> MKKHHHHHHGPEPTVEDVISQVARAHREIFTYAHDKLGSSPGNFNANHASGSPYPHGRSGRTVQEIWEDFSMSFTPAVREVVEFAKHIPGFRDLSQH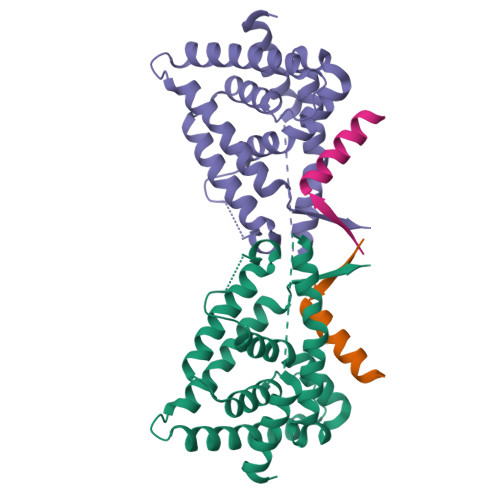DQVTLLKAGTFEVLMVRFASLFNVKDQTVMFLSRTTYSLQELGAMGMGDLLSAMFDFSEKLNSLALTEEELGLFTAVVLVSADRSGMENSASVEQLQETLLRALRALVLKNRPLETSRFTKLLLKLPDLRTLNNMHSEKLLSFRVDAQ;> THRLITLADHICQIITQDFAR methyl 6-[(5-cyanopyrazin-2-yl)amino]-4-[[(2~{R})-morpholin-2-yl]methylamino]pyridine-3-carboxylate | 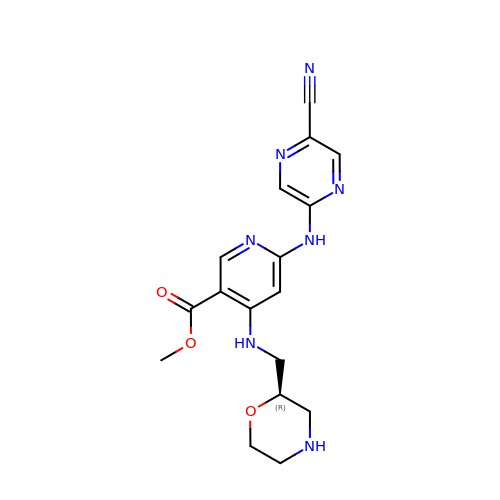C17 H19 N7 O3 | PHPWNBVMNTWSJB-GFCCVEGCSA-N>[3x]MNHKVHHHHHHLQENLYFQGMEMEAPLIVIVPSPGMGHLIPLVEFAKVLVSRFHFSVSLLLPTTAQPTKAQTTLLNSLPSSVSHNFLPTVDPAHLPDGVAHEVTISLTHAHSLSSIRAALGSLAQQAQVVALITDLF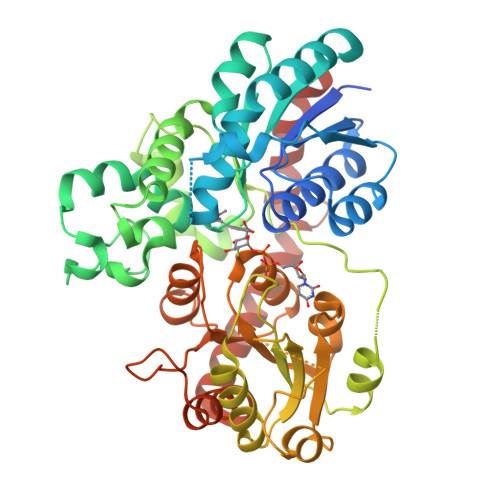GTGLYTVARDLGIPPYLYFTSTAMCLLFLFHLPKLDETVSCEYRDMPEPLVLPGCVPLHGKDFVDPAQDRQDQAYHVLLDHVKRYVLAEGIFVNTFVDLEPGAIKTLQTEDPNVPPVYPVGPIIQSGLDDDSHGSDCLKWLDRQPSGSVLFVSFGSGGTLSNEQLNELAIGLEISGHRFLWVVRSPNDHSSFGSFFSTQSQDDPFGFLPTGFVDRIKDRGLLVPSWAPQIKVLSHGSTGGFLTHCGWNSTLESIVNGVPLIVWPLYAEQRMNAVMLNQGLKVALRPNASQRGLVEADEIARVVKELMDGDEGKKARYKMRELSDSAKRVTSENGESTKLLSEVASKWSQCKS>[4x]EEKDEEFPEQKAGEVINQPMMMAARQLHDEARKWSSKGNDIIAAAKRMALLMAEMSRLVRGGSGTKRALIQCAKDIAKASDEV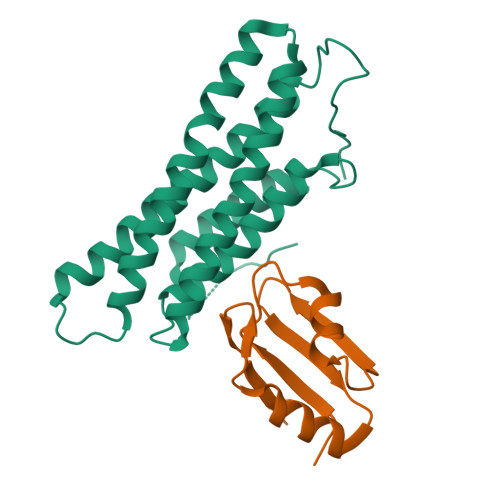TRLAKEVAKQCTDKRIRTNLLQVCERIPTISTQLKILSTVKATMLGRTNISDEESEQATEMLVHNAQNLMQSVKETVREAEAASIKIRTDAGFTLRWVRKTPWYQ;>[4x]HMRKILIRGLPGDVTNQEVHDLLSDYELKYCFVDKYKGTAFVTLLNGEQAEAAINAFHQSRLRERELSVQLQPT> KDGDQCETSPCQNQGKCKDGLGEYTCTCLEGFEGKNCELFTRKLCSLDNGDCDQFCHEEQNSVVCSCARGYTLADNGKACIPTGPYPCG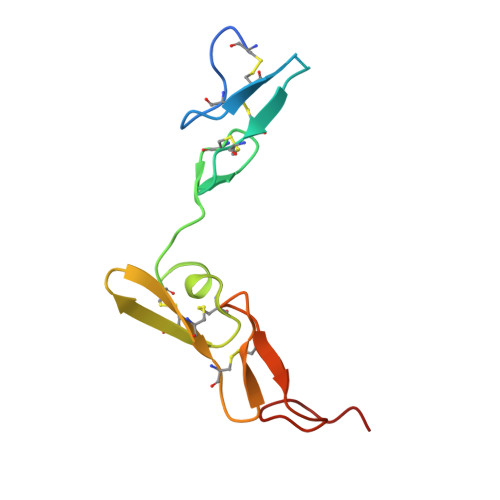KQTLE>GPIGQPVDSAVRKLLLEGAGQPFSEENIIGIYRTPLVDQQGRARFNLFQKELEATKMHRGNANVRYAWLPCSKDTMEEMMMRGVLEVTKPMLGPVYGIGTHLAPANCAQTCASYSDIDENGIMRMMLCRVIMGNVEVVLPGSKQFQPTNERFDSGVD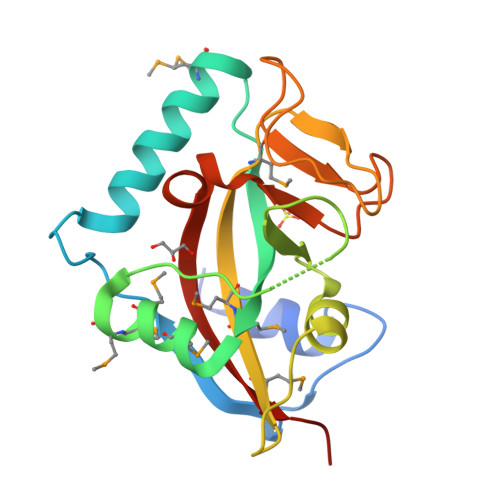DLQKPKHYIIWDANVHRHIYAEYAVVIKAPSMTN[2x]> GAGCGACCTGTACGGACA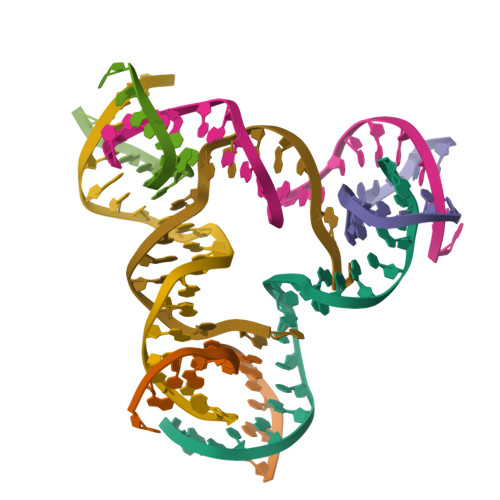TCA;> AACCTACCTGGCAGGACGACT;> CAGATACCTGATCGGACTACG;> TCTGATGTGGTAGG;> TGCGTAGTGGTCGC;> TTAGTCGTGGTATC;> CACCGATCACCTGCCAC>IRAVIYARVSSSDQKEDLERQINYLTNYATAKGYKVVEVLKDIASGLNTQRKGLLKLFKLVEGRSVDVVLITYKDRLTRFGFEYIEELFSTMGVKIEVVFGEEPKDATQELVEDLISIITSFAGKIYGMRSHKKTVLVQGVKKLIGE[4x]

TnpA binds specifically to the transposon ends and is a member of the SR family of DNA exchange enzymes, which are most often associated with site-specific recombination reactions. The SRs found in IS607-family transposable elements, however, are distinguished by the location of their DBDs at their N-termini (experimentally confirmed below). Although there is considerable structural similarity between the catalytic core domains of the subunits, the quaternary structures of the TnpA and smSRs dimers are radically different.

Although the overall configurations of the TnpAIS1535 and TnpAISC1926 dimers are similar, there are significant differences in the details of the dimer interfaces within the core. The TnpAISC1926 subunits are shifted apart by about 3 Å relative to TnpAIS1535, the TnpAISC1926 D helices are angled by about 15° rather than being parallel, and the TnpAISC1926 B helices are one turn longer than in TnpAIS1535. The active site serines of each TnpA dimer (TnpAIS1535 residue 59 and TnpAISC1926 residue 74) are separated by 28.6 and 31.5 Å (Cα atoms), respectively. The E helices are interrupted by a four residue β-turn (GRRG in TnpAIS1535 and GMRS in TnpAISC1926) and fold into an antiparallel structure. The split E helices from each subunit associate into a 4-helix bundle, with the C-terminal segments of TnpAIS1535 helix E rotated 35° relative to those of TnpAISC1926. Proteolysis experiments and structure modeling suggests that winged-helix DNA binding domains are linked to the N-terminal end of the catalytic domain by peptide chains ranging in length from just three residues to about 10 residues (IS1535). Structural models of DNA-bound TnpAISC1926 dimers, where there is predicted to be less conformational freedom between the DBD and catalytic domains, are shown in Figure 8. Thus, the two DBDs can readily fit into adjacent major groove segments on the same helical face even with the short three residue linker that is present in TnpAISC1926. The best diffracting crystals of TnpAISC1926 CTD were obtained using the hanging drop method by mixing equal volumes of a 10 mg/ml protein solution in 20 mM MOPS, pH 7.0, 100 mM Na-acetate, 0.1 mM DTT with a reservoir solution containing 8% (v/v) tacsimate, pH 4.0, and 20% (w/v) PEG3350. Crystals grew at 25°C, and although additional cryoprotectants were screened, they show no increase in diffraction relative to the drop solution alone. TnpAISC1926 CTD data were collected to 2.9 Å and integrated and scaled with XDS.Recently yeast genetics and biochemical studies indicated that the post-translational insertion of the TA proteins into ER membrane requires the co-operation of the Golgi ER trafficking (GET) complex which contains Get1, Get2 and Get3. Get3 (also named as Arr4) is the yeast homologue of TRC40 of mammals. Get3 can recognize and bind the TMD of the TA proteins. In this study, the crystal structures of Get3 from two yeast species, S. cerevisiae and D. hansenii suggest that Get3 may adopt two distinct conformations: an open conformation in nucleotide-free state and a closed conformation in ADP-bound state.

The crystal structure of S. cerevisiae full-length Get3 was determined to 2.3 Å resolution. The Get3 forms a homo-dimer (molecules A and B) in the crystal structure. In molecule A, residues 191 to 210 are missing and in molecule B, residues 93 to 116 are missing. One Magnesium ion can be located at the ATP-binding site in the NBD but no nucleotide molecules can be found even in the presence of ATP (or ADP) in the crystallization conditions. The two Get3 monomers are associated together primarily through a novel inter-molecular Zinc-finger motif, which was not previously revealed by Get3 sequence. In the crystal structure, one Zinc ion is coordinated by four Cys residues, C285 and C288 from molecule A and B, respectively. A large hydrophobic groove is found on the finger domain of Get3 structure that might represent the binding site for TMD of TA proteins. In monomer B of the Get3 dimer, a hydrophobic helix α9 from a symmetry-related Get3 monomer makes strong hydrophobic interactions with the putative TMD-binding groove. In the S. cerevisiae Get3, the two Get3 monomers are swung away from each other. The S. cerevisiae Get3 crystal structure represents the open conformation while the D. hansenii Get3 structure exhibits the closed conformation.

>[2x]MDLTVEPNLHSLITSTTHKWIFVGGKGGVGKTTSSCSIAIQMALSQPNKQFLLISTDPAHNLSDAFGEKFGKDARKVTGMNNLSCMEIDPSAALKDMNDMAVSRANNNGSDGQGDDLGSLLQGGALADLTGSIPGIDEALSFMEVMKHIKRQEQGEGETFDTVIFDTAPTGHTLRFLQLPNTLSKLLEKFGEITNKLGPMLNSFMGAGNVDISGKLNELKANVETIRQQFTDPDLTTFVCVCISEFLSLYETERLIQELISYDMDVNSIIVNQLLFAENDQEHNCKRCQARWKMQKKYLDQIDELYEDFHVVKMPLCAGEIRGLNNLTKFSQFLNKEYNPITDGKVIYELEDKE> MTGMSREEVESLIQEVLEVYPEKARKDRNKHLAVNDPAVTQSKKCIISNKKSQPGLMTIRGCAYAGSKGVVWGPIKDMIHISHGPVGCGQYSRAGRRNYYIGTTGVNAFVTMNFTSDFQEKDIVFGGDKKLAKLIDEVETLFPLNKGISVQSECPIGLIGDDIESVSKVKGAELSKTIVPVRCEGFRGVSQSLGHHIANDAVRDWVLGKRDEDTTFASTPYDVAIIGDYNIGGDAWSSRILLEEMGLRCVAQWSGDGSISEIELTPKVKLNLVHCYRSMNYISRHMEEKYGIPWMEYNFFGPTKTIESLRAIAAKFDES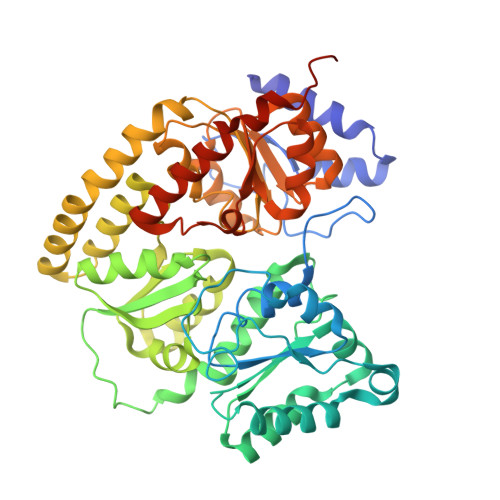IQKKCEEVIAKYKPEWEAVVAKYRPRLEGKRVMLYIGGLRPRHVIGAYEDLGMEVVGTGYEFAHNDDYDRTMKEMGDSTLLYDDVTGYEFEEFVKRIKPDLIGSGIKEKFIFQKMGIPFREMHSWDYSGPYHGFDGFAIFARDMDMTLNNPCWKKLQAPWEASEGAEKVAASA> GSGMSRREKMIAKIKDLMYKPDSIRNIGICAHIDHGKTTLSDNLLAGAGMISEELAGDQRFLDFDEQEQARGITIDAANVSMVHNYKDEEYLINLIDTPGHVDFGGDVTRAMRAVDGAVVVVCAVEGIMPQTETVLRQALKENVKPVLFINKVDRLINELKLEPEELQKRFINIYMEANKLIKNMAPEDKKEEWAVDFTDGSVAFGSAYHNWAINVPMMQETGVNFKDIIDYCNDDKQKELAQKVPL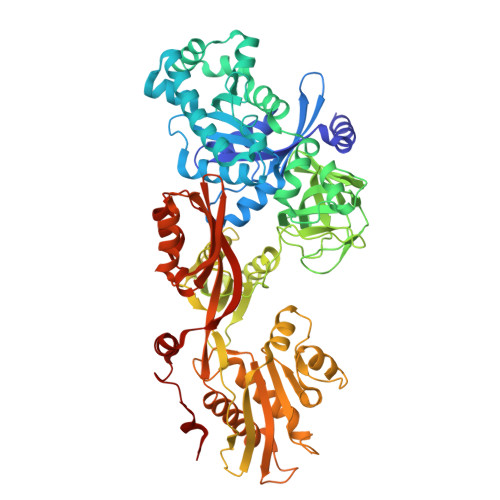SEVLLGMVVEHLPSPKVSQEYRVPNIWEGDIESPAGQGMITTSPDGPLAVMVTNVSVDKHAGEIATGRVYGGSIEKGTEVYLVGSHSKSRVQQVGVYFGPERVNTDAVPAGNIVYVAGAKGAIAGETICSPEDKIKEFEGLDHISEPVVTVAVEAKNTKDLPKLIEVLRQVAKEDPTIKVEINEETGEHLVSGMGELHLEVISYRIKDKGVEIQTSEPIVVYRETVSQLSPQVEGKSPNKHNRFYITVEPLEDELFKALQEGKLKEGKVKGKESANDFMEYGLDKEEARKVWDVYNRSVFINATRGIQYLDEVKELLIEGFESALNDGPLAKEIAMGLKFKLHDAKLHEDAVHRGPAQVLPAIRNAIYASMMSAGPTLLEPMQKVFINTPQDYMGPCTREIQNRRGQIVDMGQEGDMATIESKVPVAEMFGFAGDIRSAAEGRCLWSTEMSGFERLPREMQNQIVKEIRQRKGLSPEPYGPEHYVG> MSLRSKNSQSKPTIALYWSSDISVNIISRFLRGLQSKLAKQNYNYNVVICPYKTDCLHLEKGISKENSFDAAIIANISNYDLEYLNKASLTLPIILFNRLSNKYSSVNVDNYKMGEKASLLFAKKRYKSAAAILT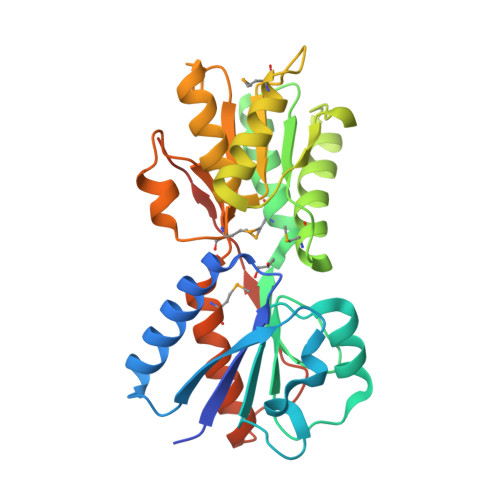ESLNDAMDNRNKGFIETCHKNGIKISENHIIAAENSIHGGVDAAKKLMKLKNTPKALFCNSDSIALGVISVLNKRQISIPDDIEIVAIGMNDREYTEFSTPPVTIVDIPIEEMAGTCISLVEKLINRDIENPTSILFDGPLILRNSEGHHHHHH> SMPVAGSELPRRPLPPAAQERDAEPRPPHGELQYLGQIQHILRCGVRKDDRTGTGTLSVFGMQARYSLRDEFPLLTTKRVFWKGVLEELLWFIKGSTNAKELSSKGVKIWDANGSRDFLDSLGFSTREEGDLGPVYGFQWRHFGAEYRDMESDYSGQGVDQLQRVIDTIKTNPDDRRIIMCAWNPRDLPLKALPPCHALCQFYVVNSELSCQLYQRSGDMGLGVPFNIASYALLTYMIAHITGLKPGDFIHTLGDAHIYLNHIEPLKIQLQREPRPFPKLRILRKVEKI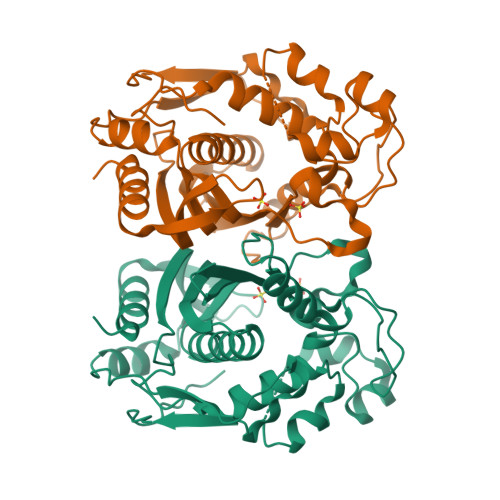DDFKAEDFQIEGYNPHPTIKMEMAV>MKSSFSGKYQLQSQENFEAFMKAIGLPEELIQKGKDIKGVSEIVQNGKHFKFTITAGSKVIQNEXTVGEECELETMTGEKVKTVVQLEGDNKLVTTFKNIKSVTELNGDIITNTMTLGDIVFKRISKRILEH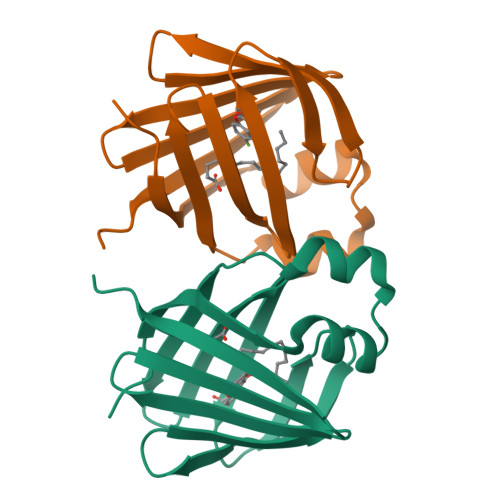HHHHH[2x]> SAEGSQACAKGCELCSEVNGCLKCSPKLFILLERNDIRQVGVCLPSCPPGYFDARNPDMNKCIKCKIEHCEACFSHNFCTK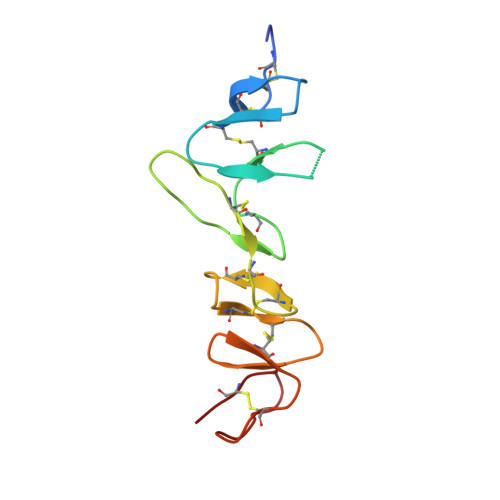CKEGLYLHKGRCYPACPEGSSAANGTMECSS> SMGKLSEQLKHCNGILKELLSKKHAAYAWPFYKPVD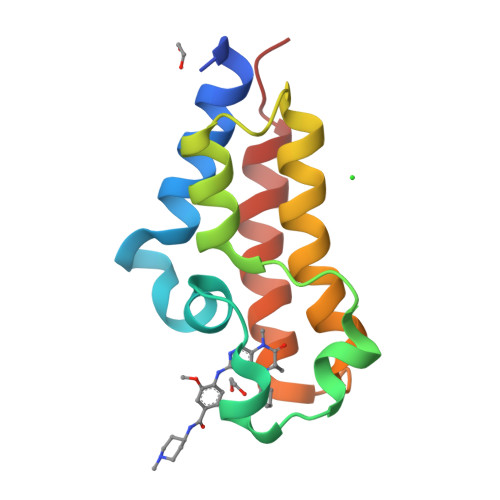ASALGLHDYHDIIKHPMDLSTVKRKMENRDYRDAQEFAADVRLMFSNCYKYNPPDHDVVAMARKLQDVFEFRYAKMPD> MTKGSLKENTIAAVLIAMTVALSILVVIPIPATKGIVTLCEVGIYTSAILYGRRMGLLVGGASGFLIDILTGYPVWCLFSLVIHGTQGLVVGWLLPRHHKGIRSMLLPLLVG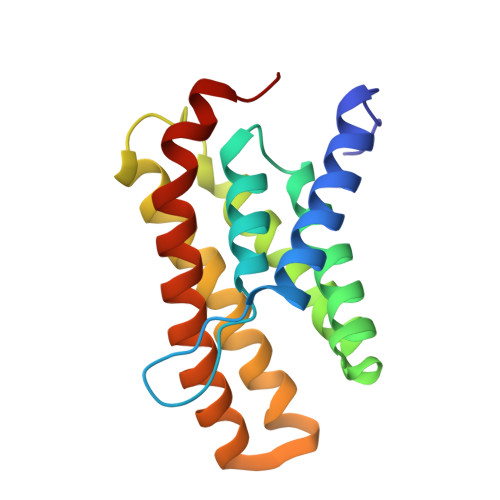SLVMVIGYCLATTLLFGWPAGLASIFGNVVQVGFGAGVTLSIVGPLTRLKPDLV> MGGSHHHHHHGMASENLYFQGGGGEIPLSSGNVNTPDVRSSGILYINIYPIVNYPETIKVSAIPYYEEFLPGKWKKRIGDLIYLYGYGIENEFDEIDNSNALFGKIFRKYLLDILSENIATPWQLKELGSTLRLVKEITENYEFSNIIKLQYELIINVHHWQNTNFGIIVDLKINILDRENNQRISYTKIKDKYGESVKKKIWVSVQAFHRHLTPEGKKYATAMRDKFNLLTGLLKEAFGSSEDEKTFSTPDGEIK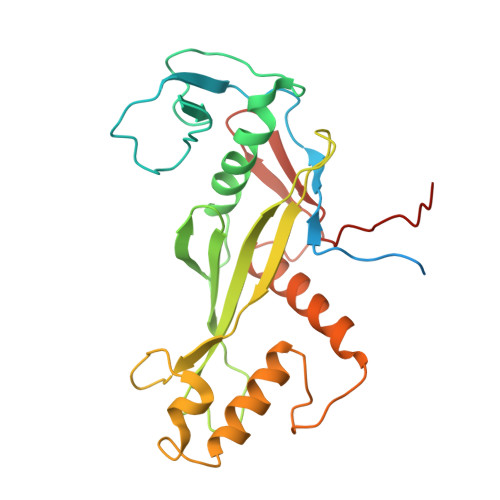IVFKPLEIVEVSNNDGI>[2x]GSHMASFLKRYTSNTYSKDEEKLIQSVSKAVQYMAKRRIGALIVFEKETGLQDYIETGIAMDSNISQELLINVFIPNTPLHDG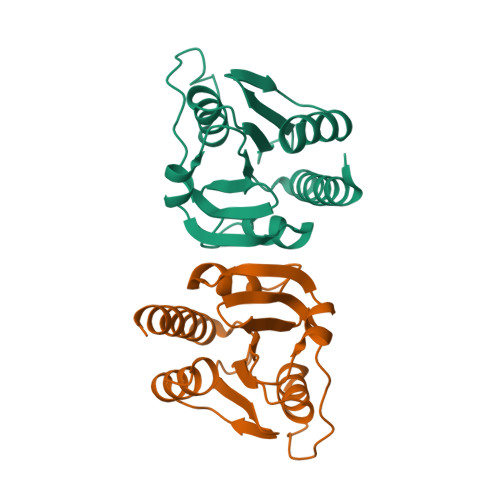AMIIQGTKIAAAASYLPLSDSPKISKSLGTRHRAAVGISEVSDAFTVIVSEETGDISVTFDGKLRRDISNEIFEELLAEHWFGTRFQKKGVK>MAKPIADD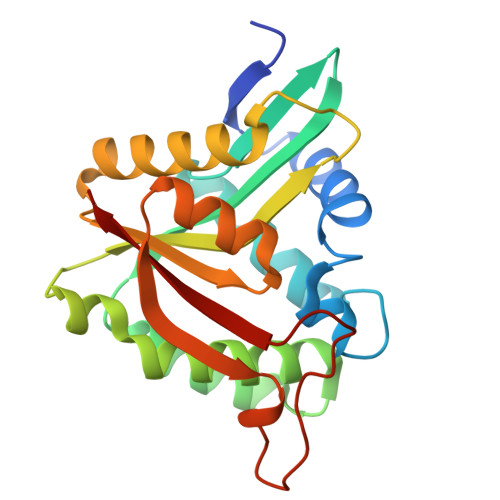IVVRQVDVGETEQLMTFLLAHYYPEEPLTAGTHPPEPEAADKEFLLSNVPFGTCFVALHEGRIVAAVVAGPKDSHEPEHMAEEARKYAGGKWGSILHLLSAVETATDVCRRFSVPSCLHVHALGVDPQLRGRNLGGRLMETVAQRGRDLGHQLVSVDCTSVYAARLVQRLGYQLINTLRYVDHLDASGQQVIRPPPPHESVQTFVLHL[2x]1-[3,5-bis(3-bromanylpropanoyl)-1,3,5-triazinan-1-yl]-3-bromanyl-propan-1-one | C12 H18 Br3 N3 O3 | 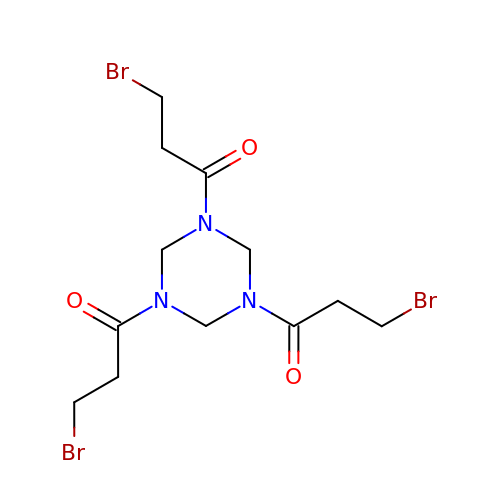UYNTZRFVDTZUQI-UHFFFAOYSA-N> MPYSVGFREADAATSFLRAARSGNLDKALDHLRNGVDINTCNQNGLNGLHLASKEGHVKMVVELLHKEIILETTTKKGNTALHIAALAGQDEVVRELVNYGANVNAQSQKGFTPLYMAAQENHLEVVKFLLENGANQNVATEDGFTPLAVALQQGHENVVAHLINYGTKGKVRLPALHIAARNDDTRTAAVLLQNDPNPDVLSKTGFTPLHIAAHYENLNVAQLLLNRGASVNFTPQNGITPLHIASRRGNVIMVRLLLDRGAQIETKTKDELTPLHCAARNGHVRISEILLDHGAPIQAKTKNGLSPIHMAAQGDHLDCVRLLLQYDAEIDDITLDHLTPLHVAAHCGHHRVAKVLLDKGAKPNSRALNGFTPLHIACKKNHVRVMELLLKTGASIDAVTESGLTPLHVASFMGHLPIVKNLLQRGASPNVSNVKVETPLHMAARAGHTEVAKYLLQNKAKVNAKAKDDQTPLHCAARIGHTNMVKLLLENNANPNLATTAGHTPLHIAAREGHVETVLALLEKEASQACMTKKGFTPLHVAAKYGKVRVAELLLERDAHPNAAGKNGLTPLHVAVHHNNLDIVKLLLPRGGSPHSPAWNGYTPLHIAAKQNQVEVARSLLQYGGSANAESVQGVTPLHLAAQEGHAEMVALLLSKQANGNLGNKSGLTPLHLVAQEGHVPVADVLIKHGVMVDATTRMGYTPLHVASHYGNIKLVKFLLQHQADVNAKTKLGYSPLHQAAQQGHTDIVTLLLKNGASPNEVSSDGTTPLAIAKRLGYISVTDVLKVVTDETSFVLVSDKHRMSFPETVDEILDVSEDEGEELISFKAERRDSRDVDEEKELLDFVPKLDQVVESPAIPRIPCAMPETVVIRSEEQEQASKEYDEDSLIPSSPATETSDNISPVASPVHTGFLVSFMVDARGGSMRGSRHNGLRVVIPPRTCAAPTRITCRLVKPQKLSTPPPLAEEEGLASRIIALGPTGAQFLSPVIVEIPHFASHGRGDRELVVLRSENGSVWKEHRSRYGESYLDQILNGMDEELGSLEELEKKRVCRIITTDFPLYFVIMSRLCQDYDTIGPEGGSLKSKLVPLVQATFPENAVTKRVKLALQAQPVPDELVTKLLGNQATFSPIVTVEPRRRKFHRPIGLRIPLPPSWTDNPRDSGEGDTTSLRLLCSVIGGTDQAQWEDITGTTKLVYANECANFTTNVSARFWLSDCPRTAEAVNFATLLYKELTAVPYMAKFVIFAKMNDPREGRLRCYCMTDDKVDKTLEQHENFVEVARSRDIEVLEGMSLFAELSGNLVPVKKAAQQRSFHFQSFRENRLAMPVKVRDSSREPGGSLSFLRKAMKYEDTQHILCHLNITMPPCAKGSGAEDRRRTPTPLALRYSILSESTPGSLSGTEQAEMKMAVISEHLGLSWAELARELQFSVEDINRIRVENPNSLLEQSVALLNLWVIREGQNANMENLYTALQSIDRGEIVNMLEGSGRQSRNLKPDRRHTDRDYSLSPSQMNGYSSLQDELLSPASLGCALSSPLRADQYWNEVAVLDAIPLAATEHDTMLEMSDMQVWSAGLTPSLVTAEDSSLECSKAEDSDATGHEWKLEGALSEEPRGPELGSLELVEDDTVDSDATNGLIDLLEQEEGQRSEEKLPGSKRQDDATGAGQDSENEVSLVSGHQRGQARITHSPTVSQVTERSQDRLQDWDADGSIVSYLQDAAQGSWQEEVTQGPHSFQGTSTMTEGLEPGGSQEYEKVLVSVSEHTWTEQPEAESSQADRDRRQQGQEEQVQEAKNTFTQVVQGNEFQNIPGEQVTEEQFTDEQGNIVTKKIIRKVVRQIDLSSADAAQEHEEVTVEGPLEDPSELEVDIDYFMKHSKDHTSTPNP;> MSSKYPRSVRRCLPLWALTLEAALILLFYFFTHYDASLEDQKGLVASYQVGQDLTVMAALGLGFLTSNFRRHSWSSVAFNLFMLALGVQWAILLDGFLSQFPPGKVVITLFSIRLATMSAMSVLISAGAVLGKVNLAQLVVMVLVEVTALGTLRMVISNIFNTDYHMNLRHFYVFAAYFGLTVAWCLPKPLPKGTEDNDQRATIPSLSAMLGALFLWMFWPSVNSPLLRSPIQRKNAMFNTYYALAVSVVTAISGSSLAHPQRKISMTYVHSAVLAGGVAVGTSCHLIPSPWLAMVLGLVAGLISIGGAKCLPVCCNRVLGIHHISVMHSIFSLLGLLGEITYIVLLVLHTVWNGNGMIGFQVLLSIGELSLAIVIALTSGLLTGLLLNLKIWKAPHVAKYFDDQVFWKFPHLAVGF;>MRFTFPLMAIVLEIAMIVLFGLFVEYETDQTVLEQLNITKPTDMGIFFELYPLFQDVHVMIFVGFGFLMTFLKKYGFSSVGINLLVAALGLQWGTIVQGILQSQGQKFNIGIKNMINADFSAATVLISFGAVLGKTSPTQMLIMTILEIVFFAHNEYLVSEIFKASDIGASMTIHAFGAYFGLAVAGILYRSGLRKGHENEESAYYSDLFAMIGTLFLWMFWPSFNSAIAEPGDKQCRAIVNTYFSLAACVLTAFAFSSLVEHRGKLNMVHIQNATLAGGVAVGTCADMAIHPFGSMIIGSIAGMVSVLGYKFLTPLFTTKLRIHDTCGVHNLHGLPGVVGGLAGIVAVAMGASNTSMAMQAAALGSSIGTAVVGGLMTGLILKLPLWGQPSDQNCYDDSVYWKVPKTR[2x];> MYGKIIFVLLLSEIVSISALSTTEVAMHTSTSSSVTKSYISSQTNGETGQLVHRFTVPAPVVIILIILCVMAGIIGTILLISYSIRRLIKA;>MYGKIIFVLLLSEIVSISASSTTGVAMHTSTSSSVTKSYISSQTNDTHKRDTYAATPRAHEVSEISVRTVYPPEEETGERVQLAHHFSEPEITLIIFGVMAGVIGTILLISYGIRRLIKKSPSDVKPLPSPDTDVPLSSVEIENPETSDQ[6x];>MEELQDDYEDMMEENLEQEEYEDPDIPESQMEEPAAHDTEATATDYHTTSHPGTHKVYVELQELVMDEKNQELRWMEAARWVQLEENLGENGAWGRPHLSHLTFWSLLELRRVFTKGTVLLDLQETSLAGVANQLLDRFIFEDQIRPQDREELLRALLLKHSHAGELEALGGVKPAVLTRSGDPSQPLLPQHSSLETQLFCEQGDGGTEGHSPSGILEKIPPDSEATLVLVGRADFLEQPVLGFVRLQEAAELEAVELPVPIRFLFVLLGPEAPHIDYTQLGRAAATLMSERVFRIDAYMAQSRGELLHSLEGFLDCSLVLPPTDAPSEQALLSLVPVQRELLRRRYQSSPAKPDS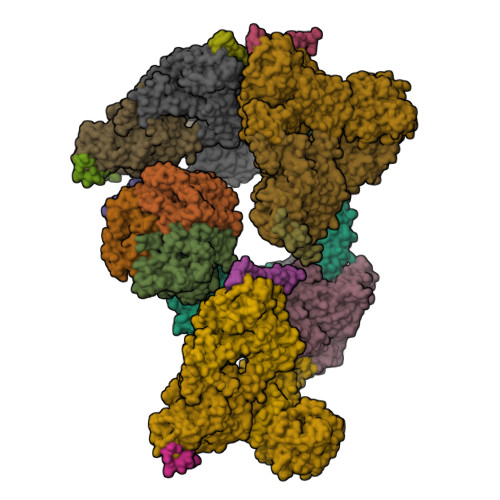SFYKGLDLNGGPDDPLQQTGQLFGGLVRDIRRRYPYYLSDITDAFSPQVLAAVIFIYFAALSPAITFGGLLGEKTRNQMGVSELLISTAVQGILFALLGAQPLLVVGFSGPLLVFEEAFFSFCETNGLEYIVGRVWIGFWLILLVVLVVAFEGSFLVRFISRYTQEIFSFLISLIFIYETFSKLIKIFQDHPLQKTYNYNVLMVPKPQGPLPNTALLSLVLMAGTFFFAMMLRKFKNSSYFPGKLRRVIGDFGVPISILIMVLVDFFIQDTYTQKLSVPDGFKVSNSSARGWVIHPLGLRSEFPIWMMFASALPALLVFILIFLESQITTLIVSKPERKMVKGSGFHLDLLLVVGMGGVAALFGMPWLSATTVRSVTHANALTVMGKASTPGAAAQIQEVKEQRISGLLVAVLVGLSILMEPILSRIPLAVLFGIFLYMGVTSLSGIQLFDRILLLFKPPKYHPDVPYVKRVKTWRMHLFTGIQIICLAVLWVVKSTPASLALPFVLILTVPLRRVLLPLIFRNVELQCLDADDAKATFDEEEGRDEYDEVAMPV[6x];> MGQALGIKSCDFQAARNNEEHHTKALSSRRLFVRRGQPFTIILYFRAPVRAFLPALKKVALTAQTGEQPSKINRTQATFPISSLGDRKWWSAVVEERDAQSWTISVTTPADAVIGHYSLLLQVSGRKQLLLGQFTLLFNPWNREDAVFLKNEAQRMEYLLNQNGLIYLGTADCIQAESWDFGQFEGDVIDLSLRLLSKDKQVEKWSQPVHVARVLGALLHFLKEQRVLPTPQTQATQEGALLNKRRGSVPILRQWLTGRGRPVYDGQAWVLAAVACTVLRCLGIPARVVTTFASAQGTGGRLLIDEYYNEEGLQNGEGQRGRIWIFQTSTECWMTRPALPQGYDGWQILHPSAPNGGGVLGSCDLVPVRAVKEGTLGLTPAVSDLFAAINASCVVWKCCEDGTLELTDSNTKYVGNNISTKGVGSDRCEDITQNYKYPEGSLQEKEVLERVEKEKMEREKDNGIRPPSLETASPLYLLLKAPSSLPLRGDAQISVTLVNHSEQEKAVQLAIGVQAVHYNGVLAAKLWRKKLHLTLSANLEKIITIGLFFSNFERNPPENTFLRLTAMATHSESNLSCFAQEDIAICRPHLAIKMPEKAEQYQPLTASVSLQNSLDAPMEDCVISILGRGLIHRERSYRFRSVWPENTMCAKFQFTPTHVGLQRLTVEVDCNMFQNLTNYKSVTVVAPELSA3'-DEAZO-THIAMIN DIPHOSPHATE | C13 H19 N3 O7 P2 S 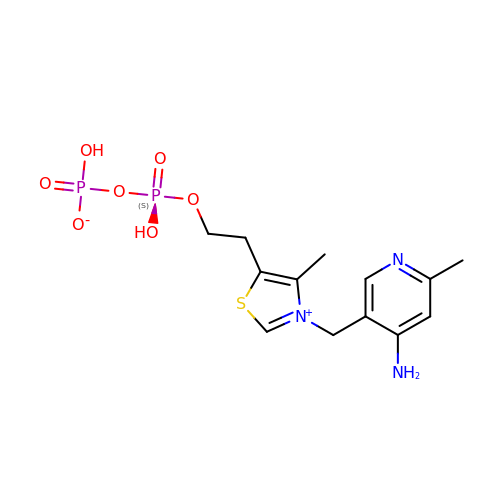| NWZZJKMZTWGIFE-UHFFFAOYSA-N(R)-(4-CARBAMIMIDOYL-PHENYLAMINO)-[5-ETHOXY-2-FLUORO-3-[(R)-TETRAHYDRO-FURAN-3-YLOXY]-PHENYL]-ACETIC 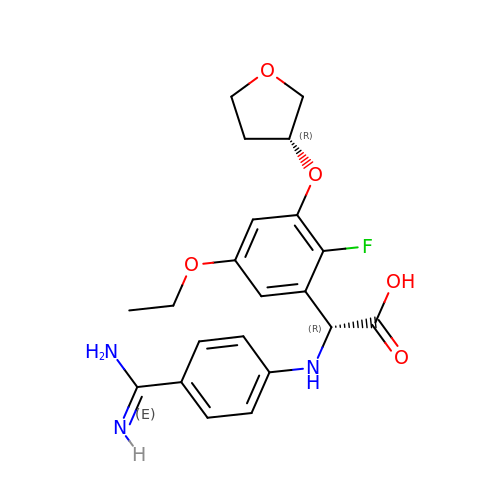ACID | C21 H24 F N3 O5 | PGYOHIAQCFZQDK-AUUYWEPGSA-N>MAFNNFIPELWSDMLLEEWTAQTVFANLV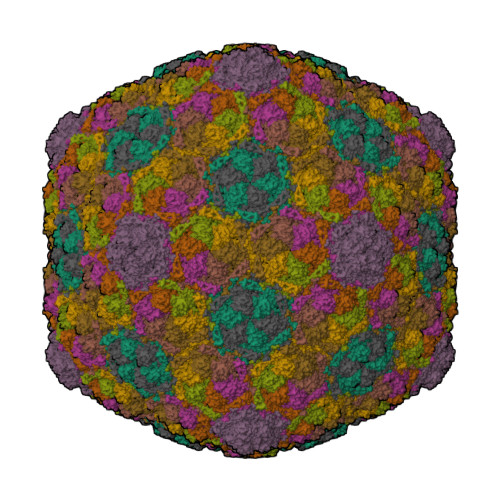NREYEGIASKGNVVHIAGVVAPTVKDYKAAGRQTSADAISDTGVDLLIDQEKSIDFLVDDIDRVQVAGSLEAYTRAGATALATDTDKFIADMLVDNGTALTGSAPSDADDAFDLIASALKELTKANVPNVGRVVVVNAEMAFWLRSSGSKLTSADTSGDAAGLRAGTIGNLLGARIVESNNLRDTDDEQFVAFHPSAAAYVSQIDTVEALRDQDSFSDRIRALHVYGGKVVRPTGVVVFNKTGS[9x]2,5-DIBROMO-3-ISOPROPYL-6-METHYLBENZO-1,4-QUINONE 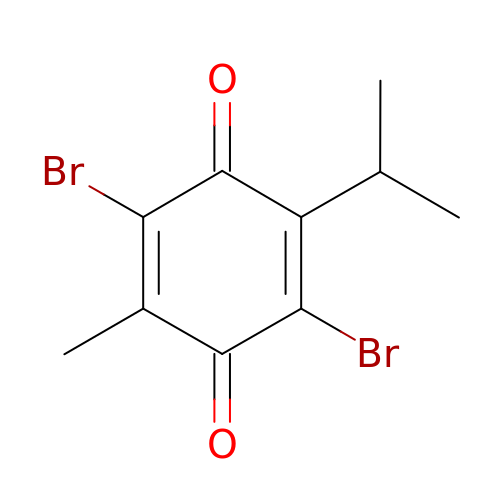| C10 H10 Br2 O2 | GHHZELQYJPWSMG-UHFFFAOYSA-N> GPVEDVITAAIGRVADTVGTGPTNSEAIPALTAAETGHTSQVVPGDTMQTRHVKNYHSRSESTVENFLCRSACVYFTEYKNSGSKRYAEWVVTTRQAAQLRRKLEFFTYIRFDLELTFVITSTQQPSTTQNQDAQILTHQIMYVPPGGPVPDKVDSYVWQTSTNPSVFWTEGNAPPRMSIPFLSIGNAYSNFYDGWSEFSRNGVYGINTLNNMGTLYARHVNTGSTGPIKSTIRIYFKPKHVKAWIPRPPRLCQYEKAKNVNFQPSGVTTTRQSITTMTNTGAF;> SPTVEECGYSDRVRSITLGNSTITTQECANVVVGYGVWPDYLKDSEATAEDQPTQPDVATCRFYTLDSVQWQKTSPGWWWKLPDALSNLGLFGQNMQYHYLGRTGYTIHVQCNASKFHQGCLLVVCVPEAEMGCATLDNTPSSAELLGGDAAKEFAGEPIASGSNKLVQRVVYNAGMGIGVGNLTIFPHQWINLRTNNSATIVMPYTNSVPMDNMFRHNNITLMVIPFVPLDYCPGSTTYVPITVTIAPMCAEYNGLRLASHQ;> GLPTMNTPGSCQFLTSDDFQSPSAMPQYDVTPEMKIPGEVKNLMEIAEVDSVVPVQNVGEKVNSMEAYQIPVRSNEGSGTQVFGFPLQPGYSSVFSRTLLGEILNYYTHWSGSIKLTFMFCGSAMATGKFLLAYSPPGAGAPTKRVDAMLG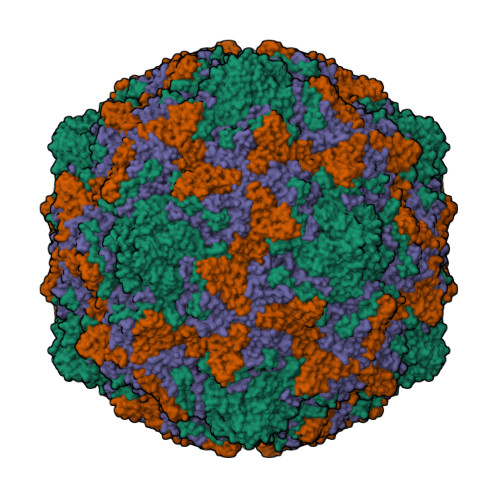THVVWDVGLQSSCVLCIPWISQTHYRYVASDEYTAGGFITCWYQTNIVVPADAQSSCYIMCFVSACNDFSVRLLKDTPFISQNSFFQ;> MGAQVSTQKTGAHETGLNASGNSIIHYTNINYYKDAASNSATRQDFAQDPGKFTEPVKDIMIKSLPALN>[4x]MRPPLIERYRNLLPVSEKTPVISLLEGSTPLIPLKGPEEARKKGIRLYAKYEGLNPTGSFKDRGMTLAVSKAVEGGAQAVACASTGNTAASAAAYAARAGILAIVVLPAGYVALGKVAQSLVHGARIVQVEGNFDDALRLTQKLTEAFPVALVNSVNPHRLEGQKTLAFEVVDELGDAPHYHALPVGNAGNITAHWMGYKAYHALGKAKRLPRMLGFQAAGAAPLVLGRPVERPETLATAIRIGNPAS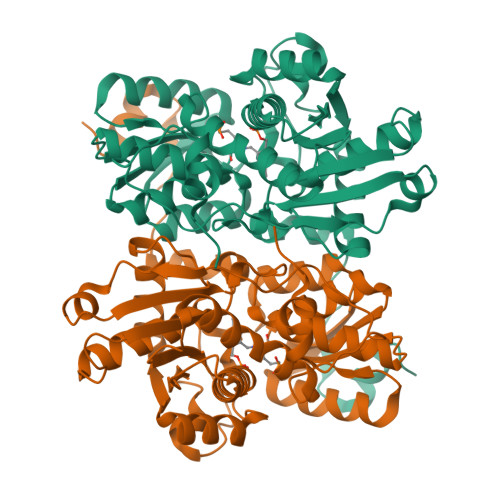WQGAVRAKEESGGVIEAVTDEEILFAYRYLAREEGIFCEPASAAAMAGVFKLLREGRLEPESTVVLTLTGHGLKDPATAERVAELPPPVPARLEAVAAAAGLL> GPMTFAVSVGGRRVDCEPGQTLLEAFLRGGVWMPNSCNQGTCGTCKLQVLSGEVDHGGAPEDTLSAEERASGLALACQARPLADTEVRSTADAGRVTHPLRDLTATVLEVADIARDTRRVLLGLAEPLAFEAGQYVELVVPGSGARRQYSLANTADEDKVLELHVRRVPGGVATDGWLFDGLAAGDRVEATGPLGDFHLPPPDEDDGGPMVLIGGGTGLAPLVGIARTALARHPSREVLLYHGVRGAADLYDLGRFAEIAEEHPGFRFVPVLSDEPDPAYRGGFPTDAFVEDVPSGRGWSGWLCGPPAMVEAGVKAFKRRRMSPRRIHREKFTPAS

As reported in a companion study, we isolated a cytochrome P450-reductase gene pair, gcoAB, from Amycolatopsis sp. ATCC 39116 (encoding proteins with accession numbers WP_020419855.1 and WP_020419854.1). Unlike other known tetrahydrofolate- or non-heme iron-dependent demethylases, which are fairly substrate specific, the P450-reductase pair characterized here (GcoAB) demethylates diverse aromatic substrates, potentially providing an important advantage in both natural and biotechnological contexts. GcoA and GcoB operate as a multi-domain complex; guaiacol is processed exclusively in GcoA, with electrons supplied by the GcoB redox machinery. While the organization of P450 systems is diverse, the architecture of this 2-protein system, combining a catalytic P450 with a 2Fe-2S ferredoxin domain in addition to FAD and NAD binding sites, represents a new class.

Analysis of the GcoB sequence, however, suggests it contains all of the necessary domains in a single polypeptide, with an N-terminal 2Fe-2S ferredoxin domain followed by an FAD and NAD(P) binding region with homology to ferredoxin-NADPH reductase (FNR) type oxido-reductases. Structurally, the compact, N-terminal 2Fe-2S domain of GcoB bears strong homology to putidaredoxin (Pdx), a ferredoxin that transfers electrons to P450cam in the three-component camphor hydroxylase system from P. putida. The C-terminal region consists of an FAD-binding domain, containing 6 beta-strands and a single alpha helix, followed by an NADH-binding domain. A structural comparison of the NADH-binding domain with the NADPH binding domain from a related CPR is strongly predictive of a binding preference for NADH over NADPH. While the individual domains are structurally similar to other CPR proteins, the overall domain architecture is not, and instead it is highly conserved with reductase proteins such as BenC27, the benzoate 1,2-dioxygenase reductase from A. baylyi ADP1, which supplies electrons to Rieske-type aromatic ring-hydroxylating dioxygenases. This suggests an unexpected convergence in the organization of the reductase partners for these evolutionarily distinct oxyenases. GcoB has an absorbance maximum at 454 nm, indicative of oxidized FAD, and peaks at 423 nm and 480 nm most likely due to the 2Fe-2S cluster. In agreement with our comparative structural analysis, the reaction with NADH was over 50-fold faster than with NADPH (kcat = 44 ± 1 s−1, KM = 16 ± 0.2 μM, 25 °C, pH 7.5; all activity measurements referenced per active cofactor). Finally, distinct from most P450 systems, the GcoB reductase is encoded as a single polypeptide rather than two.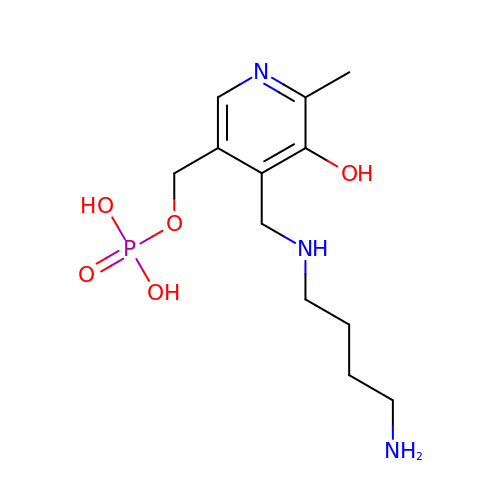(4-{[(4-AMINOBUTYL)AMINO]METHYL}-5-HYDROXY-6-METHYLPYRIDIN-3-YL)METHYL DIHYDROGEN PHOSPHATE | C12 H22 N3 O5 P | MXDZELCJRJAUEI-UHFFFAOYSA-N>MRNLKRIVMGENKLIGLVRTALDSITLGQGVNEAKIKSPQSYAFHTISVGTISLDICKAIYSSSEIGRKQLENLSKKYNMPFEDLWFYGGFLHDWNKLSGKEESLENKEELTKKIIDKLKLPNEFLHGISTMAEGHLPDNLHLPLWVSIKLADMLLISDIGSVRDVFYFANSDSYRNAIEALKEYNLELNYVSSTFRLFTLIASKELLNDVFNEKSGYFPLISYADGIVFLKRKNSQPVLLSKIVDLLSRQVFSSSSEVIEEKISDIEKCIKNKEELFRQMNIDVKSAIYDEEGKVKQINAFLPTKVCKPFEDVVGNLDNKSKLQVAREVIERNRKDIPFGLLIYFVNKFSKNEEDYIRKGLGINEKSLKYLLNIGDVQKALDKILELLEKRYAEQSSDKTLLYYVKFSSSGNIIDDLPKITDRPNDYCVVCGMPIYSSNPVRFVQYASELGGRAEIWIPREKALDEIDNVRDDWKVCPICIYEANLMKDRVKPPYFIVTFYPGVPISLLNIIDFDFSQSSIKYYIDEEKDTYFTAFEKMGGRLEPYVKKVLPAYFSSKVIIKASEVSNFSLSTRLSKSELNKLLPYAPMISMIFLTSPVLISSNLYEMPIAHERVISITSTYNYTFMKSLNSNLLTLYSIFAYSAKYDAMRKICGRSDLDNCLGYLTEEMDLYSSVDPALGVLSIGMGVGTPIDTDEKFFSAFLPVSGY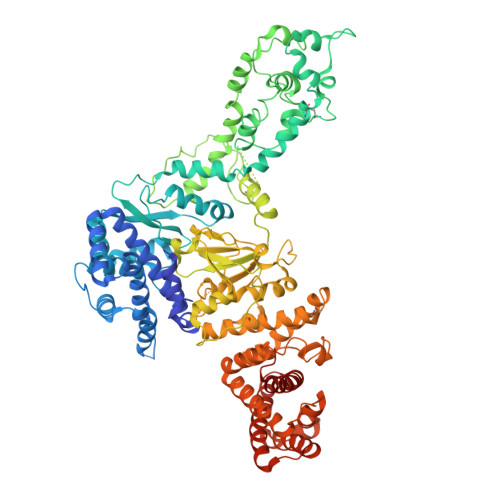LLKVTGKVSKMGETLKSSIFSIAYALKDIIKSQKVSKYDVTGFLRDGVDMFFKTTSVIKDKEDRIGISVNAAISSLENKYALDDQHRAQVYSALQDIFKTLYSIEEESDRSLAISIANTLSNWLYIAYKLVLQGDKSLEHHHHHH[2x]>[24x]SNAMIRDTATNTTQTQAAPQQAPAQQFTQAPQEKPMQSTQSQPTPSYAGTGGINSQFTRSGNVQGGDARASEALTVFTRLKEQAVAQQDLADDFSILRFDRDQHQVGWSSLVIAKQISLNGQPVIAVRPLILPNNSIELPKRKTNIVNGMQTDVIESDIDVGTVFSAQYFNRLSTYVQNTLGKPGAKVVLAGPFPIPADLVLKDSELQLRNLLIKSVNACDDILALHSGERPFTIAGLKGQQGETLAAKVDIRTQPLHDTVGNPIRADIVVTTQRVRRNGQQENEFYETDVKLNQVAMFTNLERTPQAQAQTLFPNQQQVATPAPWVASVVITDVRNADGIQANTPEMYWFALSNAFRSTHGHAWARPFLPMTGVAKDMKDIGA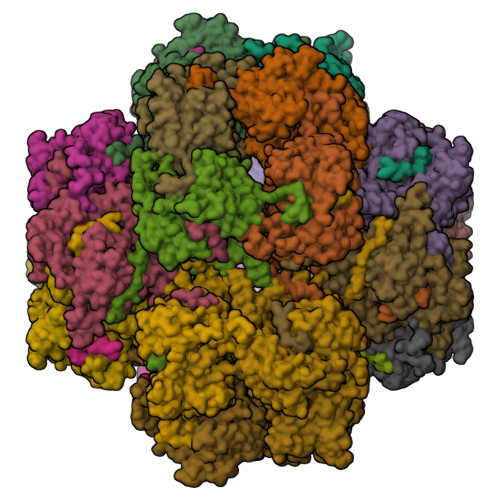LGWMSALRNRIDTKAANFDDAQFGQLMLSQVQPNPVFQIDLNRMGETAQMDSLQLDAAGGPNAQKAAATIIRQINNLGGGGFERFFDHTTQPILERTGQVIDLGNWFDGDEKRDRRDLDNLAALNAAEGNENEFWGFYGAQLNPNLHPDLRNRQSRNYDRQYLGSTVTYTGKAERCTYNAKFIEALDRYLAEAGLQITMDNTSVLNSGQRFMGNSVIGNNMVSGQAQVHSAYAGTQGFNTQYQTGPSSFY>MSQQPGVLPENMKRYMGRDAQRMNILAGRIIAETVRSTLGPKGMDKMLVDDLGDVVVTNDGVTILREMSVEHPAAKMLIEVAKTQEKEVGDGTTTAVVVAGELLRKAEELLDQNVHPTIVVKGYQAAAQKAQELLKTIACEVGAQDKEILTKIAMTSITGKGAEKAKEKLAEIIVEAVSAVVDDEGKVDKDLIKIEKKSGASIDDTELIKGVLVDKERVSAQMPKKVTDAKIALLNCAIEIKETETDAEIRITDPAKLMEFIEQEEKMLKDMVAEIKASGANVLFCQKGIDDLAQHYLAKEGIVAARRVKKSDMEKLAKATGANVITNIKDLSAQDLGDAGLVEERKISGDSMIFVEECKHPKAVTMLIRGTTEHVIEEVARAVDDAVGVVGCTIEDGRIVSGGGSTEVELSMKLREYAEGISGREQLAVRAFADALEVIPRTLAENAGLDAIEILVKVRAAHASNGNKCAGLNVFTGAVEDMCENGVVEPLRVKTQAIQSAAESTEMLLRIDDVIAAEKLRGAPDMGDMGGM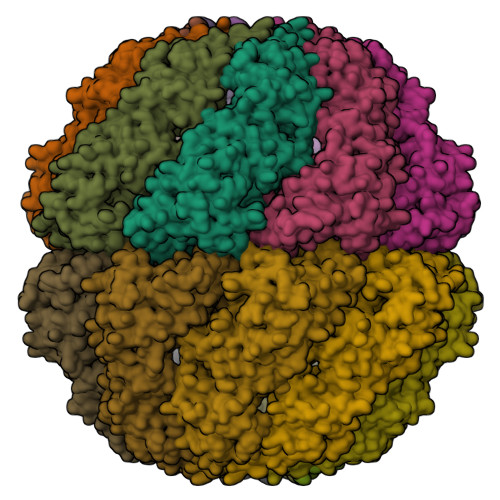PGMGGMPGMM[16x]3-phenyl-N-(5-sulfamoyl-1,3,4-thiadiazol-2-yl)propanamide 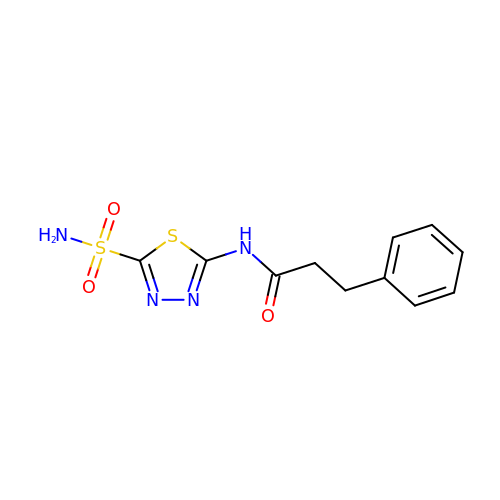| C11 H12 N4 O3 S2 | WHDSEJCOQPMZNM-UHFFFAOYSA-N> MRQSLVLLRRGKPRPRAGMFPDKYRRVPALLKPQQGGQQFFNQFLIRFTNDRLMRRDVEDGEDKKESKIAAQLPQMDWEHMSARSSSDAIREEMHRLVEGDAVQHQRVFNERIWYEEEERRRLQTGADAAAPTEDAGGAKEHDIPPRVLGNDYFQSRFGYSLVKQSEMPQGVTDYNQLDMWGEMPKYTRDMVFLYLISRRRNTYAVAYTYEGKRILSTYTAGNRGLKGGDRGFRSDGSTDNGHQVTSMYLNDLLPK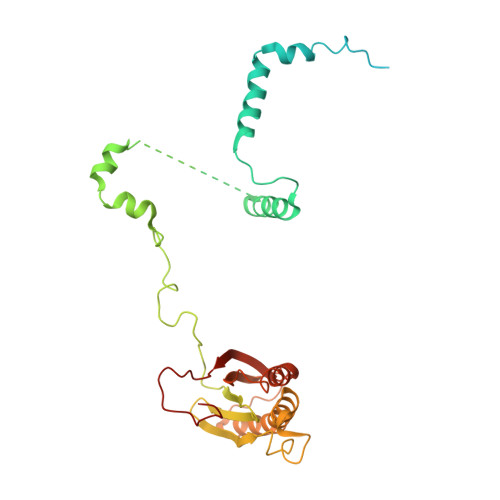VRELRANEGRPIGRGEKIELVVRVMGFYNGRQGAVRAVQDRANEFHVRYFEDITPFPLNGPKMPRGVFK>[4x]GSHNMAEMVETVCGPVPVEQLGKTLIHEHFLFGYPGFQGDVTRGTFREDESLRVAVEAAEKMKRHGIQTVVDPTPNDCGRNPAFLRRVAEETGLNIICATGYPYEGEGAPPYFQFRRLLGTAEDDIYDMFMAELTEGIADTGIKAGVIKLASS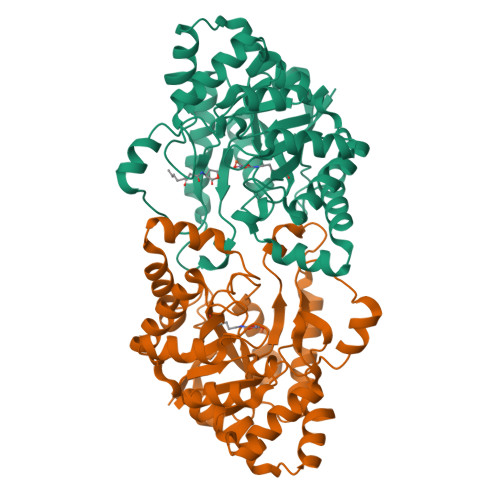KGRITEYEKMFFRAAARAQKETGAVIITHTQEGTMGPEQAAYLLEHGADPKKIVIGHMCGNTDPDYHRKTLAYGVYIAFDRFGIQGMVGAPTDEERVRTLLALLRDGYEKQIMLSHNTVNVWLGRPFTLPEPFAEMMKNWHVEHLFVNIIPALKNEGIRDEVLEQMFIGNPAALFSA N,N'-DI-1,2,3,4-TETRAHYDROACRIDIN-9-YLHEPTANE-1,7-DIAMINE | C33 H40 N4 | 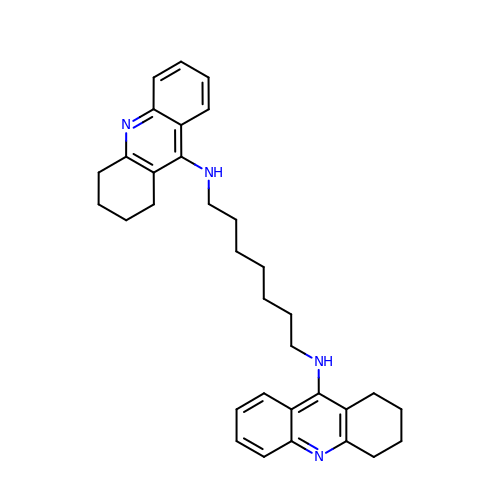ITZOKHKOFJOBFS-UHFFFAOYSA-N>[2x]MIGYLVDVEFVWGFQARIAGLSKTSPSFYYPPPTTFLGAVAEAIAKDKGIGEQRGKEIISELGENLLAIGWKALNCTPLRYS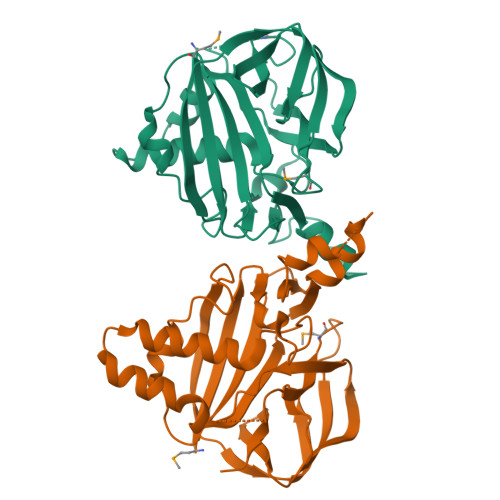DINRILAVKITSGVLYPNPQDLAKSFDSPARGKTILSSLNDEAPKIRWFLVFKEEAVEEKILWKIHRIGSKESRVAVVDVKKVKVTQKDGLISTDYSFPAEDGVELRGILSQRWEFEVYLNPFEVKYSEKENPLMSYISGKKAVLYRIPIMTSIFSTPECLVEVGGDFKAYEAGGEVVIGRCS>QELGNANFENFIGATEGFSEIAYQFTSHILTLGYAVMLAGLLYFILTIKNVDKKFQMSNILSAVVMVSAFLLLYAQAQNWTSSFTFNEEVGRYFLDPSGDLFNNGYRYLNWLIDVPMLLFQILFVVSLTTSKFSSVRNQFWFSGAMMIITGYIGQFYEVSNLTAFLVWGAISSAFFFHILWVMKKVINEGKEGISPAGQKILSNIWILFLISWTLYPGAYLMPYLTGVDGFLYSEDGVMARQLVYTIADVSSKVIYGVLLGNLAITLSKNKEL[5x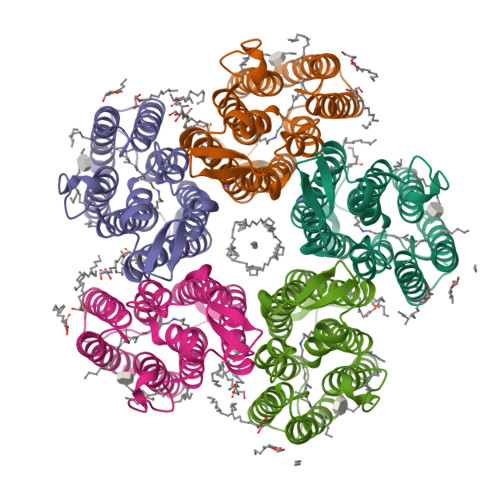]> MAQILPIRFQEHLQLQNLGINPANIGFSTLTMESDKFICIREKVGEQAQVVIIDMNDPSNPIRRPISADSAIMNPASKVIALKAGKTLQIFNIEMKSKMKAHTMTDDVTFWKWISLNTVALVTDNAVYHWSMEGESQPVKMFDRHSSLA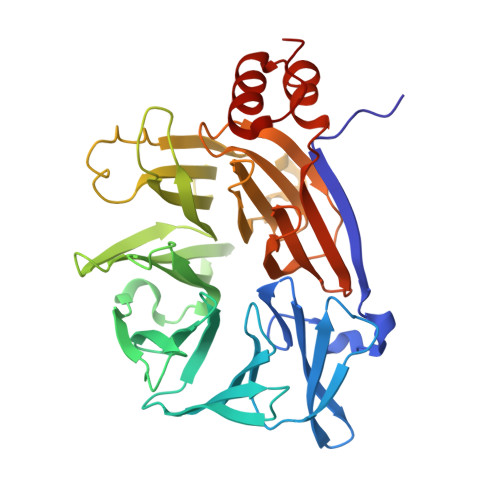GCQIINYRTDAKQKWLLLTGISAQQNRVVGAMQLYSVDRKVSQPIEGHAASFAQFKMEGNAEESTLFCFAVRGQAGGKLHIIEVGTPPTGNQPFPKKAVDVFFPPEAQNDFPVAMQISEKHDVVFLITKYGYIHLYDLETGTCIYMNRISGETIFVTAPHEATAGIIGVNRKGQVLSVCVEEENIIPYITNVLQNPDLALRMAVRNNLAGAEEL> GSHMEKNPPDDTGPVHVPLGHIVANEKWRGSQLAEEMQGKIKLIFEDGLTPDFYLSNRCCILYVTEADLVAGNGYRKRLVRVRNSNNLKGIVVVEKTRMSEQYFPALQKFTVLDLGMVLLPVASQMEASCLVIQLVQEQTKEPSKNPLLGKKRALLLSEPSLLRTVQQIPGVGK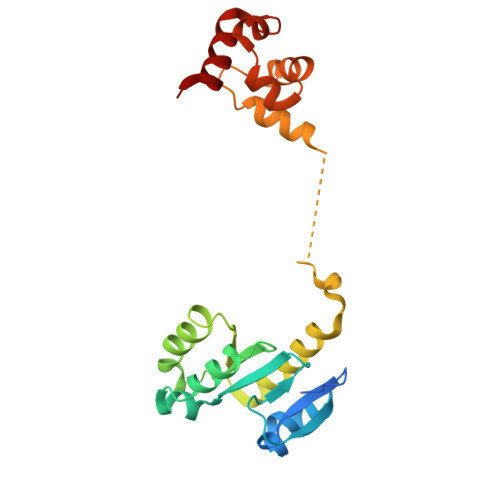VKAPLLLQKFPSIQQLSNASIGELEQVVGQAVAQQIHAFFTQP> VVGGEDAKPGQFP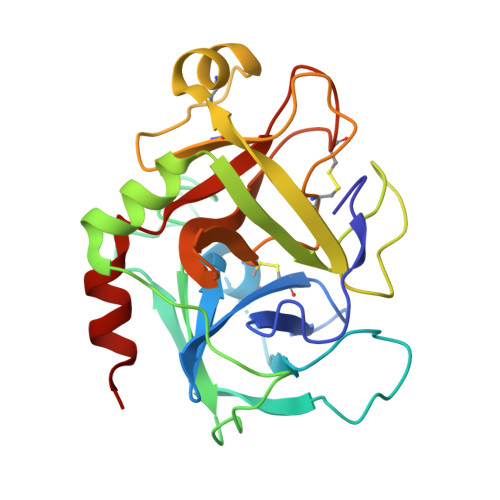WQVVLNGKVDAFCGGSIVNEKWIVTAAHCVETGVKITVVAGEHNIEETEHTEQKRNVIRIIPHHNYNAAINKYNHDIALLELDEPLVLNSYVTPICIADKEYTNIFLKFGSGYVSGWGRVFHKGASALVLQYLRVPLVDRATCLRSTKFTIYNNMFCAGFHEGGRDSCQGDSGGPHVTEVEGTSFLTGIISWGEECAMKGKYGIYTKVSRYVNWIKEKTKLT> MTSLIDLGRYVERTHHGEDTEPRSKRVKIAKPDLSSFQPGSIIKIRLQDFVTYTLTEFNLSPSLNMIIGPNGSGKSTFVCAVCLGLAGKPEYIGRSKKVEDFIKNGQDVSKIEITLKNSPNVTDIEYIDARDETIKITRIITRSKRRSDYLINDYQVSESVVKTLVAQLNIQLDNLCQFLSQERVEEFARLKSVKLLVETIRSIDASLLDVLDELRELQGNEQSLQKDLDFKKAKIVHLRQESDKLRKSVESLRDFQNKKGEIELHSQLLPYVKVKDHKEKLNIYKEEYERAKANLRAILKDKKPFANTKKTLENQVEELTEKCSLKTDEFLKAKEKINEIFEKLNTIRDEVIKKKNQNEYYRGRTKKLQATIISTKEDFLRSQEILAQTHLPEKSVFEDIDIKRKEIINKEGEIRDLISEIDAKANAINHEMRSIQRQAESKTKSLTTTDKIGILNQDQDLKEVRDAVLMVREHPEMKDKILEPPIMTVSAINAQFAAYLAQCVDYNTSKALTVVDSDSYKLFANPILDKFKVNLRELSSADTTPPVPAETVRDLGFEGYLSDFITGDKRVMKMLCQTSKIHTIPVSRRELTPAQIKKLITPRPNGKILFKRIIHGNRLVDIKQSAYGSKQVFPTDVSIKQTNFYQGSIMSNEQKIRIENEIINLKNEYNDRKSTLDALSNQKSGYRHELSELASKNDDINREAHQLNEIRKKYTMRKSTIETLREKLDQLKREARKDVSQKIKDIDDQIQQLLLKQRHLLSKMASSMKSLKNCQKELISTQILQFEAQNMDVSMNDVIGFFNEREADLKSQYEDKKKFVKEMRDTPEFQSWMREIRSYDQDTKEKLNKVAEKYEEEGNFNLSFVQDVLDKLESEIAMVNHDESAVTILDQVTAELRELEHTVPQQSKDLETIKAKLKEDHAVLEPKLDDIVSKISARFARLFNNVGSAGAVRLEKPKDYAEWKIEIMVKFRDNAPLKKLDSHTQSGGERAVSTVLYMIALQEFTSAPFRVVDEINQGMDSRNERIVHKAMVENACAENTSQYFLITPKLLTGLHYHEKMRIHCVMAGSWIPNPSEDPKMIHFGETSNYSFD;> MISTTISGKRPIEQVDDELLSLTAQQENEEQQQQRKRRRHQFAPMTQFNSNTLDEDSGFRSSSDVATADQDNFLEESPSGYIKKVILRNFMCHEHFELELGSRLNFIVGNNGSGKSAILTAITIGLGAKASETNRGSSLKDLIREGCYSAKIILHLDNSKYGAYQQGIFGNEIIVERIIKRDGPASFSLRSENGKEISNKKKDIQTVVDYFSVPVSNPMCFLSQDAARSFLTASTSQDKYSHFMKGTLLQEITENLLYASAIHDSAQENMALHLENLKSLKAEYEDAKKLLRELNQTSDLNERKMLLQAKSLWIDVAHNTDACKNLENEISGIQQKVDEVTEKIRNRQEKIERYTSDGTTIEAQIDAKVIYVNEKDSEHQNARELLRDVKSRFEKEKSNQAEAQSNIDQGRKKVDALNKTIAHLEEELTKEMGGDKDQMRQELEQLEKANEKLREVNNSLVVSLQDVKNEERDIQHERESELRTISRSIQNKKVELQNIAKGNDTFLMNFDRNMDRLLRTIEQRKNEFETPAIGPLGSLVTIRKGFEKWTRSIQRAISSSLNAFVVSNPKDNRLFRDIMRSCGIRSNIPIVTYCLSQFDYSKGRAHGNYPTIVDALEFSKPEIECLFVDLSRIERIVLIEDKNEARNFLQRNPVNVNMALSLRDRRSGFQLSGGYRLDTVTYQDKIRLKVNSSSDNGTQYLKDLIEQETKELQNIRDRYEEKLSEVRSRLKEIDGRLKSTKNEMRKTNFRMTELKMNVGKVVDTGILNSKINERKNQEQAIASYEAAKEELGLKIEQIAQEAQPIKEQYDSTKLALVEAQDELQQLKEDINSRQSKIQKYKDDTIYYEDKKKVYLENIKKIEVNVAALKEGIQRQIQNACAFCSKERIENVDLPDTQEEIKRELDKVSRMIQKAEKSLGLSQEEVIALFEKCRNKYKEGQKKYMEIDEALNRLHNSLKARDQNYKNAEKGTCFDADMDFRASLKVRKFSGNLSFIKDTKSLEIYILTTNDEKARNVDTLSGGEKSFSQMALLLATWKPM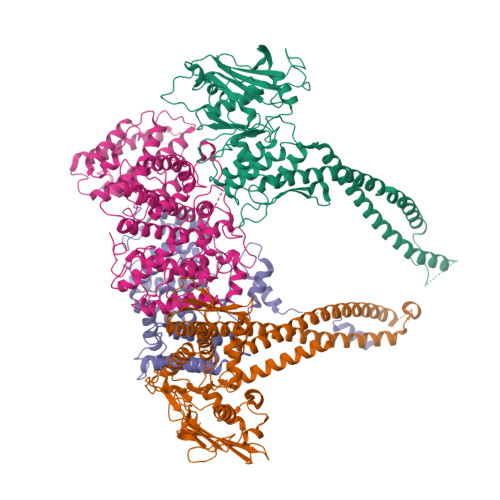RSRIIALDEFDVFMDQVNRKIGTTLIVKKLKDIARTQTIIITPQDIGKIADIDSSGVSIHRMRDPERQNNSNFYN;> MGSVNSSPNEEFETVPDSQISGFDSPLIPTSVGSYFRDDDDDEKVHPNFISDPENDSLNSDEEFSSLENSDLNLSGAKAESGDDFDPILKRTIISKRKAPSNNEDEEIVKTPRKLVNYVPLKIFNLGDSFDDTITTTVAKLQDLKKEILDSPRSNKSIVITSNTVAKSELQKSIKFSGSIPEIYLDVVTKETISDKYKDWHFISKNCHYEQLMDLEMKDTAYSFLFGSSRSQGKVPEFVHLKCPSITNLLVLFGVNQEKCNSLKINYEKKENSRYDNLCTIFPVNKMLKFLMYFYSDDDNDDVREFFLKAFICLILDRKVFNAMESDHRLCFKVLELFNEAHFINSYFEIVDKNDFFLHYRLLQIFPHLQSALLRRRFSEKQGRTETIQQNIIKEFNEFFDCKNYKNLLYFILTMYGSKFIPFGPKCQVTEYFKDCILDISNETTNDVEISILKGILNLFSKIR;> MDGALINSVLYVSPRNGAHYFVELTEKHLLAFEMLNSMCLLENYDHVLLFLECQFGKSHNLAVIPFDIILVLFTLSTLSEYYKEPILRANDPYNTSRETLSRRALKLLQKYLAILKEFDSEQYNLYDLELLRCQFFLAIDTLTPKKQKWGFDRFRRTKSESGVTYRQNASVDPELDQAKTFKNPYRSYISCLEQRNTILGNRLLNLKLNEPGEFINMILWTLSNSLQESTPLFLSSHEIWMPLLEILIDLFSCRQDYFIQHEVAQNVSKSLFVQRLSESPLAVFFESLNTRNFANRFSEYVFLNCDYKLPSDNYATPVHPVYNGENTIVDTYIPTIKCSPLYKSQKSLALRRKLIGSCFKLLLRVPDGHRLITPRIVADDVIQGISRTLASFNDILQFKKFFMTENLSQESYFIPLLAEGTLSEILKDTQECVVILTLVENLSDGVSFCNEVIGLVKSKCFAFTEQCSQASYEEAVLNIEKCDVCLLVLLRYLLHLIGTEAILDAKEQLEMLHAIEKNDSGRRQWAKALNLGNDPPLLYPIVSQMFGVHDKSVIIE> XXXXXXXXXXX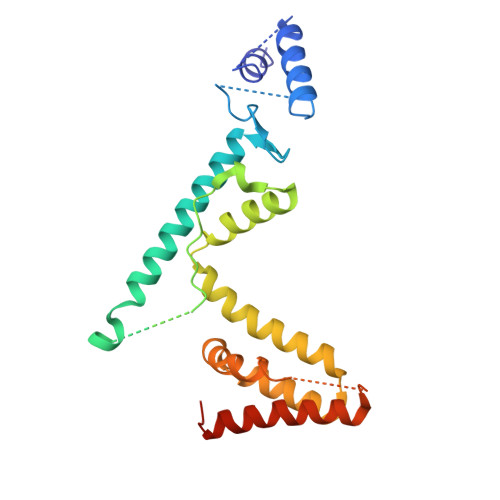XXXXXXXXXXXXXXXXXXXXXXXANMRYQFEKNAYGVVASKAKIAEIERNTKEVQRLVDEKIKAMKDKEYYAGGKPQGTIEQRIAMTSPAHVTGINRPHDFDFSKVRSYSRLRTLEESMEMRTDPQYYEKKMIQLQLNFIKSVEGSFNSFDAADELIEELKKIPPDDFYELFLRISEISFEEFDSEGNTVENVEGNVYKILSYLEQYRRGDFDLSLKGF IMIDAZO[1,2-A]PYRIDINE | C7 H7 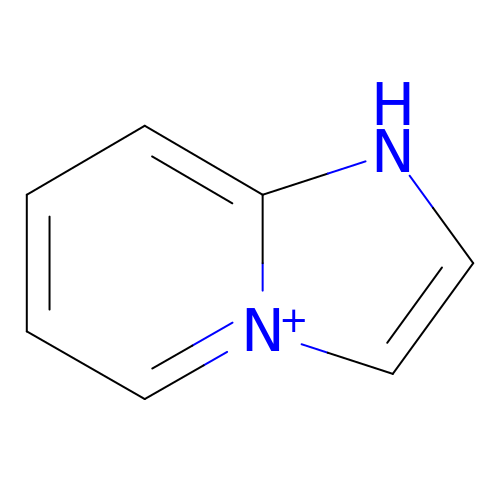N2 | UTCSSFWDNNEEBH-UHFFFAOYSA-O F-type ATP synthases are energy-converting membrane protein complexes that synthesize adenosine triphosphate (ATP) from ADP and inorganic phosphate. These universal enzymes function by using the energy stored in an electrochemical potential across the bioenergetic membrane by rotary catalysis. In mitochondria, F1Fo ATP synthase resides in the crista membrane where it is known to form dimers, which can further assemble into rows critical for inducing the membrane curvature and maintaining membrane potential and morphology. Here, we investigate the mechanism for the generation of the unique cristae in the Apicomplexa, using a combination of single-particle cryo-EM, cryo-ET and subtomogram averaging.

The IF1-arrested structure, in which ATP synthases are locked in a single rotational state, allowed us to obtain a map of the rotor-stator interface at 3.5 Å, resolving both the c-ring and H5-6 of subunit-a, where proton transfer occurs. In addition, unlike in the canonical six-helix (H1-6a) fold, which is conserved in bacteria, chloroplasts and other mitochondria, the subunit-a in T. gondii lacks H1-4a, and only the horizontal H5a and H6a are found. They interact with the c-ring at the rotor-stator interface. Mechanistically, the essential arginine on H5a (Arg166 in T. gondii) is thought to be responsible for deprotonation of the conserved glutamate on the c-ring (Glu150 in T. gondii). Our structure indicates that in the open conformation Glu150 is within 2.3 Å distance from the juxtaposed Arg166, allowing the formation of a salt bridge. The rotor-stator interface surrounding the Arg166/Glu150 pair is more hydrophobic compared to other structures, with subunits a and c contributing a total of eight aromatic residue side chains. Thus, the tight hydrophobic interface between the decameric c-ring and subunit-a in T. gondii is consistent with a direct, rather than water-mediated Arg/Glu interaction. The apicomplexan-conserved Fo-subunit ATPTG11 extends from the lumenal region and plugs the central cavity of the c-ring. This is mediated by the short N-terminal amphipathic helix of ATPTG11 (Ala9-Leu17), which is sequence-conserved in Apicomplexa. The interface is located on the border of the detergent belt and dominated by hydrophobic residues of ATPTG11 pointing towards the inside of the c-ring, which is unlikely to inhibit the rotation of the rotor.

>[10x]MFFSRLSLSALKAAPAREALPGLLSRQSFSSAGFSQFSSQKFFFSPSRNFSQSPLFQKHTPVHCNQRIASALVPTQQPAMTRQNPYAMQVGARYDAGVASLSAAIALMSVGGVAQGIGSLFAALVSGTARNPSIKEDLFTYTLIGMGFLEFLGIICVLMSAVLLYS;> MAAGSRFPFCTAARLSSRGTLPRLGEATFFAGAESQRSAGAFAKTLQRPFLRAPSTQLFPVGNRLGVSSARALVANAMEPRRFFAAAASAKATHALQPTGTGSVAFTRPGQGSNAQFQTSLADKTRGLLGVGFLRPTKMASFAATFLLNFRFYFMYMARTTFQAVRPLLAFSVFGEVMKLVLATMSSGLFSFLFSFVLAFEVFYFFLQCYISYTFLTMFFTVLF;> MVRNQRYPASPVQEIFLPEPVPFVQFDQTAPSPNSPPAPLPSPSLSQCEEQKDRYRDISSMFHRGVAGAEQVREAYNSMAKCFRRVSVAEVLESDPAFRQARNFTMDLKQAEDDQRYKQLQYGRVPSILTKYHL;> MFARAFSRFASLAAPAPQRGWNAFVLPSRHFATAAGGANPFKNQLLLTLSSPSEAIYVRTPVRSVTVPGSEGAMTMTNGHSQTVARLKAGEIIVRKGETGDEVERFFLSDGFVLFKSPEDDSGCCTAEVLGVEVVPVSMLDKESAATALQELLQQGAGATDEWTKARTLLGQELLSSVIRAAP;> MWRSSGVSFTRYASEMAALLRQCLKEPYRTQAMQRNQIHLKETVYQQGQVLTRETFNDIKKAFEAAAKHAGEK;> MAGLASLSSVGALRGMRLVPAAHLLPLHSAFGQQTRNFGAGDLKIVAARMKSVKSIQKITKAMKMVAASKLRMDQRRLENGLPFATPVQKLVQRIPVDPKEKGTLAVLALSSDKGLCGGVNSFVAKQARIVIKENEMAGNAVQVYGVGDKIRSALQRTFGDRFKRIMTEVTRFPWNFGQACIIADRLMQDNPARLMVIYNHFKSAVAYDTLTLNVLTPTQAAQSAKEQLNTFEFEPEKTDVWKDLQDFYYACTVFGCMLDNIASEQSARMSAMDNASTNAGEMISSLTLRYNRARQAKITTELVEIISGANALE> GDPIADMIDQTVNNQVNRSLTALQVLPTAANTEASSHRLGTGVVPALQAAETGASSNASDKNLIETRCVLNHHSTQETAIGNFFSRAGLVSIITMPTTGTQNTDGYVNWDIDLMGYAQLRRKCELFTYMRFDAEFTFVVAKPNGELVPQLLQYMYVPPGAPKPTSRDSFAWQTATNPSVFVKMTDPPAQVSVPFMSPASAYQWFYDGYPTFGEHLQANDLDYGQCPNNMMGTFSIRTVGTEKSPHSITLRVYMRIKHVRAWIPRPLRNQPYLFKTNPNYKGNDIKCTSTSRDKITTL;> MGSQVSTQRSGSHENSNSASEGSTINYTTINYYKDAYAASAGRQDMSQDPKKFTDPVMDVIHEMAPPLKSPSAEACGYSDRVAQLTIGNSTITTQEAANIVIAYGEWPEYCPDTDATAVDKPTRPDVSVNRFFTLDTKSWAKDSKGWYWKFPDVLTEVGVFGQNAQFHYLYRSGFCVHVQCNASKFHQGALLVAVLPEYVLGTIAGGTGNENSHPPYATTQPGQVGAVLTHPYVLDAGIPLSQLTVCPHQWINLRTNNCATIIVPYMNTVPFDSALNHCNFGLLVIPVVPLDFNTGATSEIPITVTIAPMCAEFAGLRQAVKQ;> GIPTELKPGTNQFLTTDDGVSAPILPGFHPTPPIHIPGEVHNLLEICRVETILEVNNLKTNETTPMQRLCFPVSVQSKTGELCAAFRADPGRDGPWQSTILGQLCRYYTQWSGSLEVTFMFAGSFMATGKMLIAYTPPGGNVPADRITAMLGTHVIWDFGLQSSVTLVVPWISNTHYRAHARAGYFDYYTTGIITIWYQTNYVVPIGAPTTAYIVALAAAQDNFTMKLCKDTEDIEQTANIQ

Enterovirus 71 (EV71) and coxsackievirus A16 (CVA16) are subgroup A human enteroviruses (HEVA), small, nonenveloped single-stranded RNA (ssRNA) viruses whose protective capsid mediates cell entry and humoral immune responses. The external portion of the icosahedral capsid comprises 60 copies of viral proteins VP1, -2, and -3 arranged with pseudo T=3 symmetry, while their N-terminal extensions and 60 copies of VP4 line the interior, surrounding the RNA genome. There is a “canyon” (a depression encircling the 5-fold axes) on the surface of enteroviruses that often harbors the receptor binding site, and there is a fatty acid binding site below the canyon base, within the hydrophobic β-barrel core of VP1. Here, we remedy this with high resolution X-ray structures of both mature and natural empty CVA16 particles and also of empty recombinant viruslike particles of CVA16 produced in insect cells, a potential vaccine antigen.

VLPs were secreted from Sf9 insect cells infected with recombinant baculovirus containing the P1 and 3CD genes of CVA16 (09-7 strain) and purified by ultracentrifugation. Crystals of CVA16 VLPs diffracted to 2.5 Å. The space group of CVA16 VLP crystals is P4232, with unit cell dimensions of: a = b = c = 347 Å. The recombinant CVA16 capsid is self-assembled from VP0, VP1, and VP3. This particle is unexpanded and in the native antigenic state, and thus, the external surface of the VLP is structurally indistinguishable from the mature virus and natural empty particles (RMSD in Cα atoms of 0.4 Å and 0.3 Å, respectively). As expected, the residues lining the inner surface of the particle show more disorder; indeed, they seem a little more disordered than those of the natural empty particle. Disordered residues include residues 8 to 23 and 36 to 61 of VP1 and residues 1 to 13, 46 to 64, and 77 to 81 of VP0. Residues 65 to 76 of VP0, which include the cleavage site between 69 and 70 (cleavage of which produces VP4 and VP2) are well defined in the density. The pocket factor binding site located inside the β-barrel of VP1 is fully occupied by a fatty acid acquired from the Sf9 insect cells, which differs somewhat from that derived from mammalian cells and is modeled as stearic acid. Compared to the head group in CVA16 mature and empty particles, the smaller carboxyl head group of the stearic acid is positioned about 3 Å lower than the hydroxyl oxygen of the sphingosine and forms a hydrogen bond to the main chain nitrogen of Leu113, similar to the carbonyl oxygen of the sphingosine.> PLGSMS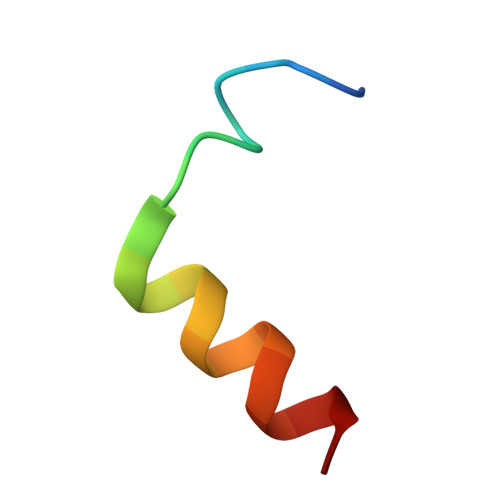RIKNWGDEVEEQEMRT> MAVDSSNSATGPMRVFAIGNPILDLVAEVPSSFLDEFFLKRGDATLATPEQMRIYSTLDQFNPTSLPGGSALNSVRVVQKLLRKPGSAGYMGAIGDDPRGQVLKELCDKEGLATRFMVAPGQSTGTCAVLINEKERTLCTHLGACGSFRIPENWTTFASGALIFYATAYTLTA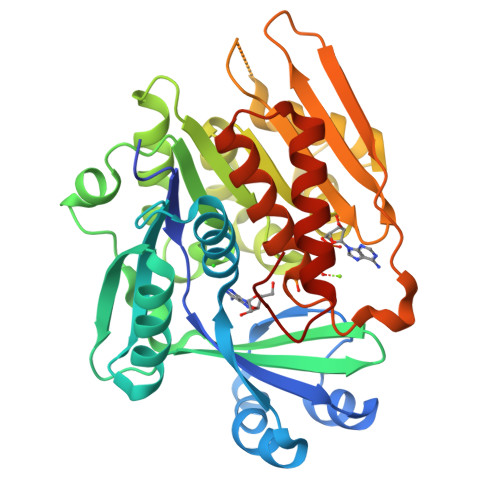TPKNALEVAGYAHGIPNAIFTLNLSAPFCVELYKDAMQSLLLHTNILFGNEEEFAHLAKVHNLVAAEKVALSVANKEHAVEVCTGALRLLTAGQNTGATKLVVMTRGHNPVIAAEQTADGTVVVHEVGVPVVAAEKIVDTNGAGDAFVGGFLYGLSQGKTVKQCIMCGNACAQDVIQHVGFSLSFTSLPC>[4x]MWHTHSEREKRVSNA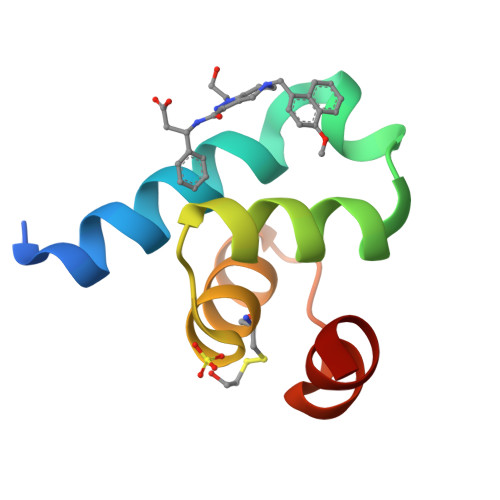VEFLLDSRVRRTPTSSKVHFLKSKGLSAEEICEAFTKVGQPKTLNEIKRILS> MSLKWSAIPFQTLYRSIESGEFDFDLFKEVLPDLQNLNLNTDKLKNNASRSQLEKGEIELSDGSTFKVNQEFIFEAISLSDELNLDEIVACELILSGDTTANNGKVQYFLRRQYILQIVSFIVNCFHEDTELYQELIKNGALVSNILSAFKFIHTQLSEIKQQINKAQILENYNALFQQNIKFRRDFLLREYDILSQILYGLVDKGAIMKNKDFILSLLHHVSELDSNDFFIIYYTPAFFHLFASLRVLPDADVKLLHSQFMKDLKDDSIYTKPVKVALIFIFFAYFIGWCKEDPKRRADTMDFKTDVDEPMTSAVELGAIEQILIFAADTSIVEQDKSMELFYDIRSLLERHIPRLIPKQLLDDEKIFSQTTNSTYNPASATDNMSGRGLWNPSYPGMMSTTGTARLNSMPNNVNEYSYTTIVLSDQTQEFFLSSFDDVLQTIITDCAFLLTKIKDAEEDSLLSGEDLTLDDISLKADLERFFLSIYFFYASRPEYSCTFWSDKESNAYGFIEWCSRCNDNLMRSCFYLMVSSLSFGPENALNVYHYFGENSSISWKNIAQCLSDYTKKISNFNSSLHKRQQFSESTHNDIDSTAVALEEGLNEEAVIFLSSLLTLVGSVTYQVDEDVKSSLSKVFSDVLFEFTKINTPLVGAAFKVISNLVPKLESSRTKFWSFLDSLIFKDSSLNYSSESYRNAFTNVLTKYSDVLGFLQLFHNLISIHSRENNSEYMVFGKLAFPTRLGQGYRKVGIWPYFDYIFNDILAHVDQIVDIRNKRAVQLPILKIIYTGLCSFDYSVILNSIPAAANLDALVDCENFFNYVQECPAIPIFNYIFTEKIYKSIFNVVDVGVDQLSIELEGGKNQAELLQLAVKIINKVLDYQETYVEELFPIVKKHGKTDYFLPKNYSLHGLRSFYDAIFFNIPLVAHLGLYVGVDDQILATNSLRIL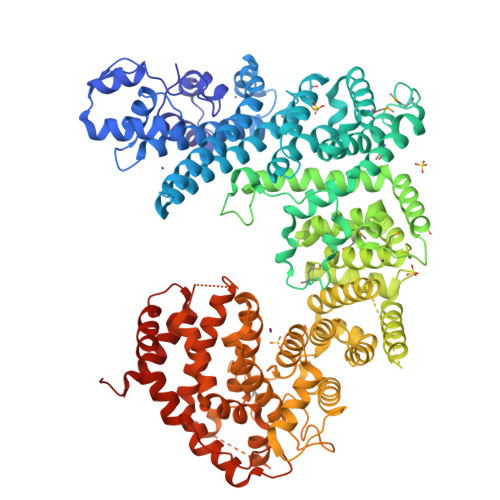AKLSERSNGSVASLSEGHHHHHH> ADLTASTTVTVTVVEPARITLTYKEGAPITIMDNGNIDTELLVGTLTLGGYKTGTTSTSVNFTDAAGDPMYLTFTSQDGNNHQFTTKVIGKDSRDFDISPKVNGENLVGDDVVLATGSQDFFVRSIGSKGGKLAAGKYTDAVTV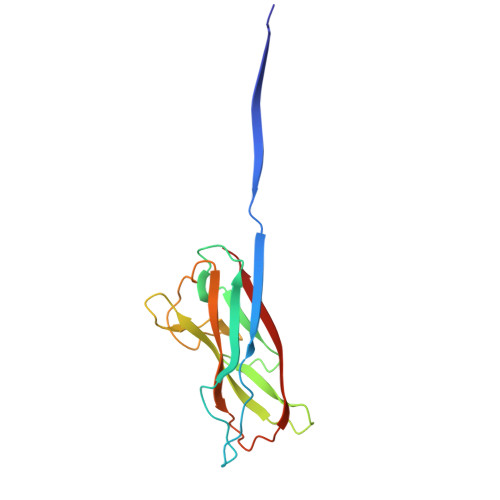TVSNQ Here, we explain the mechanism by which the phage AR9 non-virion RNAP (nvRNAP), a bacterial RNAP homolog, recognizes the −10 element of its deoxyuridine-containing promoter in the template strand. The AR9 sigma-like subunit, the nvRNAP enzyme core, and the template strand together form two nucleotide base-accepting pockets whose shapes dictate the requirement for the conserved deoxyuridines. The catalytically active AR9 nvRNAP core enzyme consists of four proteins that, when pairwise concatenated, show about 20% sequence identity and cover the entire lengths of the universally conserved β and β′ subunits of bacterial RNAPs. Promoter-specific transcription is performed by a five-subunit holoenzyme that, in addition to the nvRNAP core, contains the product of AR9 gene 226 (gp226).

The structure of the promoter complex has been determined by both X-ray crystallography and cryo-EM to resolutions of 3.38 and 3.80 Å, respectively. Where required, we will distinguish the X-ray and cryo-EM-derived structures of the AR9 nvRNAP promoter complex by referring them as AR9 nvRNAP-Pro-Xray and AR9 nvRNAP-Pro-cryoEM, respectively. In the most populous class of the cryo-EM reconstruction and in both available crystal forms of the AR9 nvRNAP promoter complex (i.e., AR9 nvRNAP-Pro-cryoEM and AR9 nvRNAP-Pro-Xray), the enzyme bound not one but two copies of the P077 promoter-containing forked oligonucleotide—the downstream copy (as designed) and (fortuitously) the upstream one—resulting in a superstructure that resembles the complete transcription bubble found in open complexes formed by other RNAPs. In the structure of the same complex analyzed by cryo-EM, only three nucleotides of the promoter (3′-−11UGU−9-5′) were sufficiently ordered for model building. The −8U nucleotide is partially disordered in the AR9 nvRNAP-Pro-cryoEM map. The cryo-EM- and X-ray-derived structures of the holoenzyme in the promoter complex were very similar and could be superimposed with a root mean square deviation (RMSD) of 1.84 Å between 2563 and 97% of all Cα atoms comprising the holoenzyme. Although weak, the X-ray electron density and cryo-EM map of the upstream oligonucleotide stretches from the σ2-like part of the gp226 NTD to the gp226 CTD.

> MDILENYVSFDEQARDINIAFDKLFGRDDISHMNNFSINKRSYYNCLDQISDDLNLVLNKYNDLAYSLLEIRYNMATKENYTHMEFYSDIERLFIKNEKLLNVISDIVEEEYDLDLNQASKGKKINIELQVTDNLNKIYLKSSVLMRILIPILCDFNCDDDINEVLVYDIFKEVIKSFDDGKKNALNKLYKIIYSRVFETKYSDVVIWTYLKNMSTDLMIIVKDYFKVIIKKIFPKLKHNSSVISYLDVVIKQKLKYLFTFKYPISYKPLKAETTDDEELSEQERMEINLLRNDQGNSIINECSIKQEIAKIKKKYNVTDEVMKEFINGRELNSIQIYLVKIYYSNKFKVNSNKNDIFYLLYGMTRELGEMNFSIIPEILSCAIAPNVRKMNNRKKLVDKIIHSDKYSYLLKSYLPIKNILDKNNVILQLMTIKNAKFMNKENKEVDFSTDHLAEEVLDMLLCI;> MDDISVIKNEDYEGSHRFLAEELLMPNANKTDGNRSTMFCSHLAQAVTLQKAEPPLVYTNFENQVGKYSTAGYRKANSNYKVIEKIYKNDYNYVLIVQDQETGEYTLFERAECEFLTEHYGFQWDNDKIDSLKKDDTIEKDTVLYKNTCYDENMNFGYGVNLNAAYFSYKNETLEDAIVISESAAKKLGTFSVNKVKVSVNTNDILLNLYGDNENYKGFPDIGEHIKNQIIASRRRFDYNTALYELKNLNEMRDSDTPFFADGKIVDIEIFSNVPEEELKVQKYNEQVLYYINKQKEFSNNVYQKLKKIVEGKDNNVSDKLLHFYNNCKMRIDENISYTYQNSKFSGFIMEFTILEEEPLNKGSKITGRYGNKGVISKILPDDQMPTVAEGRFKGLKADICLNPLGVFNRLNPSQLIEQELNWIAKFIRKDMEEAGSNEEKVSILLDFLNRVNKEETELMEEFINSLNKTELEEFLNDIIENGIPICQKPFFGNIGLDELWELYNHYDHIDYFKCEGISTPLIIGEIYMVRLKHEPHSKFSARSTSFMNLRGLPAKSKNFKEHKDLYSKTPVRIGNMEISNLSLTNEMGSIMDMLNSYSNNETNRRELIMQLLTGNPFDTNIDLSDVESGTSKILKSLFTCLGLSIDDVEEEWENKLNGKVEDEK;> MEKTYNLNDILLSNEYEKIKEDIKEEIINDMASKKVKYSNTSEFAKNDFLKDEFIDLVVDGETYEITYGNLITLLIVARPFNHFKVPMTEDLLFDLSDLKEYQNYYTTLLEHFGYSNEIKSIIKDVISELAIFSGDINVTFGNTVSIKSLIDLGNKVKRFRELLHYRLPNDEALEFNDIEAIIKKNLDEIMKILSETDNMLRYYIDSGAGINSKQFGQVLSLVGSKPDLFGKIIPYPINTSFLRGLDVRSFYINALGARKALITNYQQVRNSGYLTRKISMLLMDTKLIDLDDCGSHENNYLSINVENKDVLKRFSKRSYLNNNGELVEIDINDESLIGQVIKIPSPTTCASNEGVCRKCYGKLFDINKDLNIGMIAVLLLTDPLTQRLLSAKHLLETRSSKIDWGTNFEENFIVNRNLIYPKVYNGTVIIKEDDFKEDEETEEQVFDTFTLKSGNRFISISSPMRLFLNKDLKKQLDESFYNIEEMQFEIPLNKLDEGDSFATFIMDNNELSKPLREIKDLIETNKYIKDHNVNEVVNYFIYLLNESGINIQSVHSELIIREMMKLDDSDRTQFKNDKMPDYEIFRITDANLKGDSLSRSLLFEQVKKQLTTLDYDTFNKTKSSILDKLL;> MISNFRKFHGNKNQEKFNENLILNKENESILNYLDPICKTLEIIPEITYLGSSVEPINKVYKFNKEEKTSDIERSELQLIKMSFLIEKDDKKEEINKFIYFPKLIDSQYFIINGNRYYPIYQLLDSGTYRTNKALTLKTLLMPIVLREKKETFDDINGETHTMLNVDLDLFKSKVPFLIYFFSKFGFEGTLEYFGLQDLIHVLMKEDLDQLDEDEINDNVIFMITKNISLVVDKNFFSNKNNQIIIATLLNCFNTRIKIDKIYEKDYWVKKLGGYFTTNNSNKQEKGEGIILSFERILDEWTKKILRTEEKNKEDIYSVVRWMINNYLALVKQDNMNLANKRIRLYEYLLHPLLIKFSKGTYRVLNNRNSNKFEKIKTIFSNIQEGFLVKKIINNELLRYDNSVNSISLFTLILRYTQSGPQSPFSSNSTNNKLRGLHPSYLGRLGLTSTSAGDPGASGSLTPFLELPENSYMHFTEEPEINLNIDDISIDEVIES;> MGSSHHHHHHSSGENLYFQGHHMGKKLSLIDFNEIYNEENLITRANPIENHEFSDDGIYSERIFGSYNEDDDDKDIDTIGWINIEPYYIINPILFTIIKKCIPSINKIINYQQSIDQNGENIDLTEEIGEDDYIGLVKFKDNFDDLLEKYTDKKKYQKEYDFLIENHDKIFINKLPVFSHKLRPATLLTGSKGKVLAFDEINNYYNFVIEYINQINEGVVSDDSIDLLLLPLLYNMQFYANNILTRIISEYLRGKKGFLRKNIMGSRINFSARNVITPLIGHPIDEVAMPYKTFAELYKFQLINLISKVKGINYNEALKFWEKGILGFNQELYNYMEELITKTKGGCTFLLNRNPTISIGSILYLKIGLIKKDYKDLTLGISNNLLSALSGDYDGDVLNIIPVFDNKMKEHFSLLSPQNFLVDRNNGRFNGDFDLQKDQILGIFILNN> FEKVELTADGGVIKTILKKGDEGEENIPKKGNEVTVHYVGKLESTGKVFD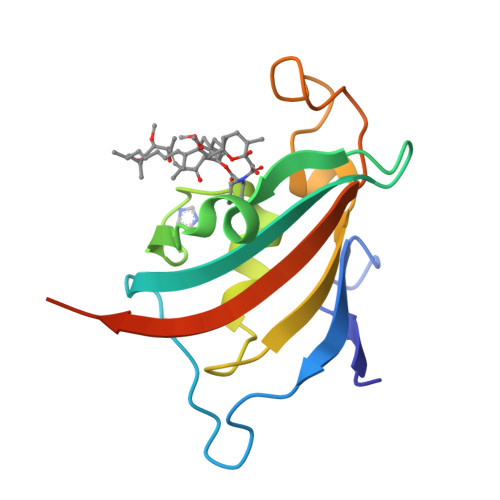SSFDRNVPFKFHLEQGEVIKGWDICVSSMRKNEKCLVRIESMYGYGDEGCGESIPGNSVLLFEIELLSFRELETSHHHHHH> MAATTVNGGTVHFKGEVVNAACAVDAGSVDQTVQLGQVRTASLAQEGATSSAVGFNIQLNDCDTNVASKAAVAFLGTAIDAGHTNVLALQSSAAGSATNVGVQILDRTGAALTLDGATFSSETTLNNGTNTIPFQARYFATGAATPGAANADATFKVQYQ;> MGVALGATRVIYPAGQKQEQLAVTNNDENSTYLIQSWVENADGVKDGRFIVTPPLFAMKGKKENTLRILDATNNQLPQDRESLFWMNVKAIPSMDKSKLTENTLQLAIISRIKLYYRPAKLALPPDQAAEKLRFRRSANSLTLINPTPYYLTVTELNAGTRVLENALVPPMGESTVKLPSDAGSNITYRTINDYGALTPKMTGVMEHHHHHH;> DLYFNPRFLADDPQAVADLSRFENGQELPPGTYRVDIYLNNGYMATRDVTFNTGDSEQGIVPCLTRAQLASMGLNTASVAGMNLLADDACVPLTTMVQDATAHLDVGQQRLNLTIPQAFMSNRARGYIPPELWDPGINAGLLNYNFSGNSVQNRIGGNSHYAYLNLQSGLNIGAWRLRDNTTWSYNSSDRSSGSKNKWQHINTWLERDIIPLRSRLTLGDGYTQGDIFDGINFRGAQLASDDNMLPDSQRGFAPVIHGIARGTAQVTIKQNGYDIYNSTVPPGPFTINDIYAAGNSGDLQVTIKEADGSTQIFTVPYSSVPLLQREGHTRYSITAGEYRSGNAQQEKPRFFQSTLLHGLPAGWTIYGGTQLADRYRAFNFGIGKNMGALG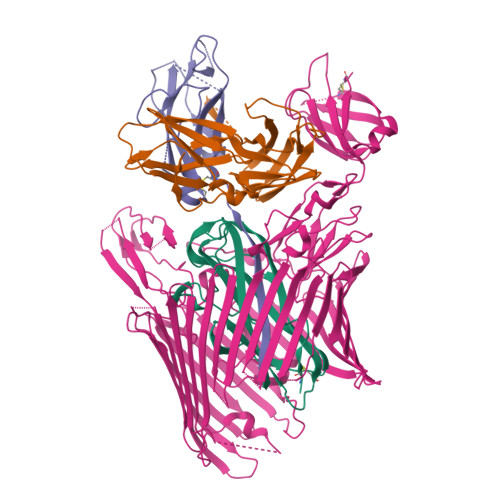ALSVDMTQANSTLPDDSQHDGQSVRFLYNKSLNESGTNIQLVGYRYSTSGYFNFADTTYSRMNGYNIETQDGVIQVKPKFTDYYNLAYNKRGKLQLTVTQQLGRTSTLYLSGSHQTYWGTSNVDEQFQAGLNTAFEDINWTLSYSLTKNAWQKGRDQMLALNVNIPFSHWLRSDSKSQWRHASASYSMSHDLNGRMTNLAGVYGTLLEDNNLSYSVQTGYAGGGDGNSGSTGYATLNYRGGYGNANIGYSHSDDIKQLYYGVSGGVLAHANGVTLGQPLNDTVVLVKAPGAKDAKVENQTGVRTDWRGYAVLPYATEYRENRVALDTNTLADNVDLDNAVANVVPTRGAIVRAEFKARVGIKLLMTLTHNNKPLPFGAMVTSESSQSSGIVADNGQVYLSGMPLAGKVQVKWGEEENAHCVANYQLPPESQQQLLTQLSAECRLVPRGSWSHPQFEK;> GNKWNTTLPGGNMQFQGVIIAETCRIEAGDKQMTVNMGQISSNRFHAVGEDSAPVPFVIHLRECSTVVSERVGVAFHGVADGKNPDVLSVGEGPGIATNIGVALFDDEGNLVPINRPPANWKRLYSGSTSLHFIAKYRATGRRVTGGIANAQAWFSLTYQ3-[3-chloro-5-(trifluoromethyl)pyridin-2-yl]-2-methyl-1H-indole 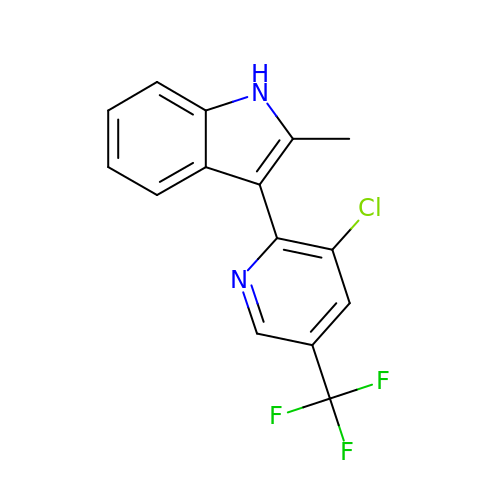| C15 H10 Cl F3 N2 | DFUZKSKLYCWMQD-UHFFFAOYSA-N> GPLGSGRPMEVLFEAKVG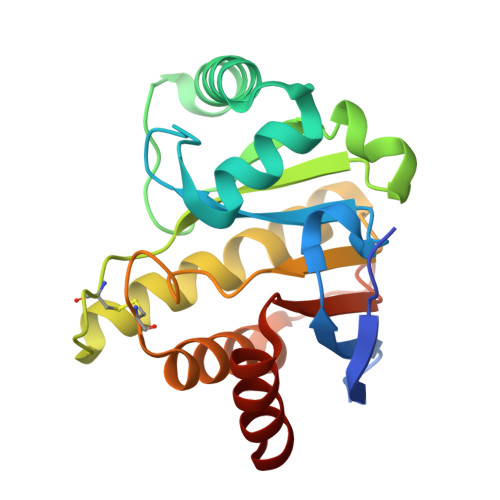DITLKLAQGDITQYPAKAIVNAANKRLEHGGGVAYAIAKACAGDAGLYTEISKKAMREQFGRDYIDHGEVVVTPAMNLEERGIKYVFHTVGPICSGMWSEELKEKLYKAFLGPLEKAEEMGVESIAFPAVSAGIYGCDLEKVVETFLEAVKNFKGSAVKEVALVIYDRKSAEVALKVFERSL> MEYKSSPKRPYLLRAYYDWLVDNSFTPYLVVDATYL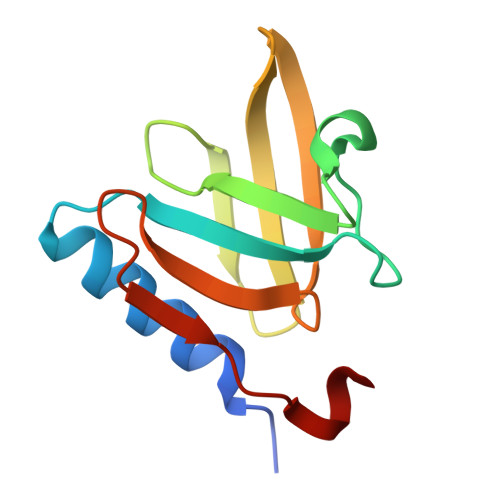GVNVPVEYVKDGQIVLNLSASATGNLQLTNDFIQFNARFKGVSRELYIPMGAALAIYARENGDGVMFEPEEIYD> SMPQALSTDILIVGGGIAGLWLNARLRRAGYATVLVESASLGGGQSVKSQGIIHGGAKYALHGALTGASEAIADMPRRW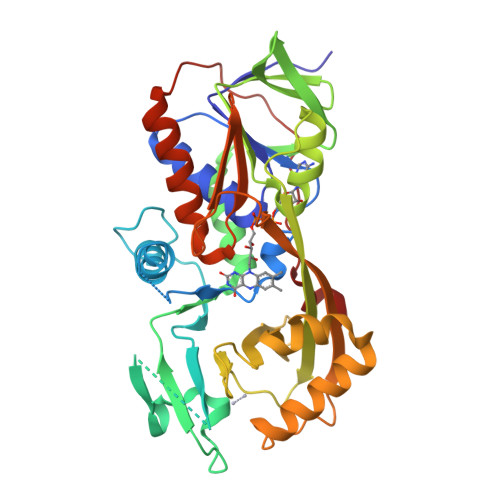RACLGSDGELDLRGVRLLSEAHYLWSPGGLAGSLTSFFASKAVRSRVEQAKGEDLPPALRDKGFKGKAYRLTEIVFDVPDLIRRLAELAGDSLLAGERIEPLREGRELAGLCVDGREIRAQRVVLSAGAGNEALLRELGLEQPAMQRRPLHMVMVKAATLKPLYAHCLGAGPKPRITVTTHPTRDGQSVWYLGGDIAETDGVARDEAAQIAEARRELAKLLPWIDLGQAQWATLRVDRAEPAQSNLLRPDNAFLAEQGRLLVGWPTKLALAPDFADRVCARLEEDGIRPSEHAALPQLPRPPLAEPAWEVAFA N-(2-ethoxy-4-{5-[({[(2R)-2-{(1R)-1-[formyl(hydroxy)amino]propyl}heptanoyl]amino}methyl)carbamoyl]furan-2-yl}benzene-1-carbonyl)-L-aspartic 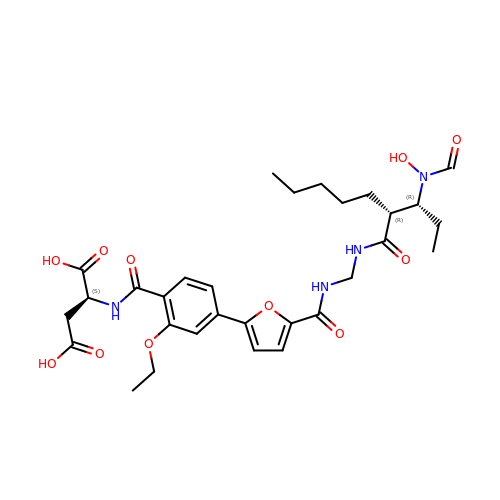acid | C30 H40 N4 O11 | SFAJGGFDBDWTMC-BAGYTPMASA-N>[7x]MTMFQYYKRSRHFVFSAFIAFVFVLLCQNTAFARASSNGDLPTKADLQAQLDSLNKQKDLSAQDKLVQQDLTDTLATLDKIDRIKEETVQLRQKVAEAPEKMRQATAALTALSDVDNDEETRKILSTLSLRQLETRVAQALDDLQNAQNDLASYNSQLVSLQTQPERVQNAMYNASQQLQQIRSRLDGTDVGETALRPSQKVLMQAQQALLNAEIDQQRKSLEGNTVLQDTLQKQRDYVTANSARLEHQLQLLQEAVNSKRLTLTEKTAQEAVSPDEAARIQANPLVKQELEINQQLSQRLITATENGNQLMQQNIKVKNWLERALQSERNIKEQIAVLKGSLLLSRILYQQQQTLPSADELENMTNRIADLRLEQFEVNQQRDALFQSDAFVNKLEEGHTNEVNSEVHDALLQVVDMRRELLDQLNKQLGNQLMMAINLQINQQQLMSVSKNLKSILTQQIFWVNSNRPMDWDWIKAFPQSLKDEFKSMKITVNWQKAWPAVFIAFLAGLPLLLIAGLIHWRLGWLKAYQQKLASAVGSLRNDSQLNTPKAILIDLIRALPVCLIILAVGLILLTMQLNISELLWSFSKKLAIFWLVFGLCWKVLEKNGVAVRHFGMPEQQTSHWRRQIVRISLALLPIHFWSVVAELSPLHLMDDVLGQAMIFFNLLLIAFLVWPMCRESWRDKESHTMRLVTITVLSIIPIALMVLTATGYFYTTLRLAGRWIETVYLVIIWNLLYQTVLRGLSVAARRIAWRRALARRQNLVKEGAEGAEPPEEPTIALEQVNQQTLRITMLLMFALFGVMFWAIWSDLITVFSYLDSITLWHYNGTEAGAAVVKNVTMGSLLFAIIASMVAWALIRNLPGLLEVLVLSR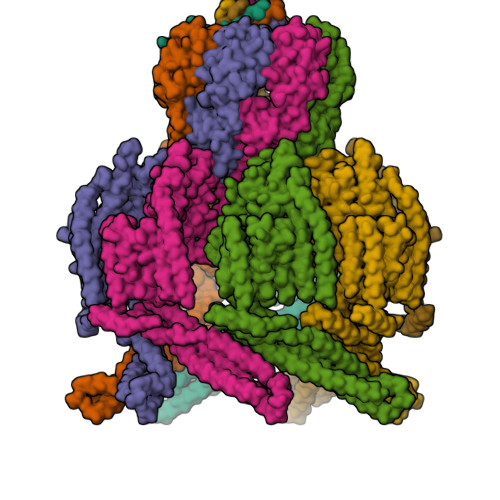LNMRQGASYAITTILNYIIIAVGAMTVFGSLGVSWDKLQWLAAALSVGLSFGLQEIFGNFVSGLIILFERPVRIGDTVTIGSFSGTVSKIRIRATTITDFDRKEVIIPNKAFVTERLINWSLTDTTTRLVIRLGVAYGSDLEKVRKVLLKAATEHPRVMHEPMPEVFFTAFGASTLDHELRLYVRELRDRSRTVDELNRTIDQLCRENDINIAFNQLEVHLHNEKGDEVTEVKRDYKGDDPTPAVG> SVSFYEIANGNEVHTGSLNMTANPTSHELNVSAVLAAAKAKYAAHQLENGASNGASVAVTTDVKDLTDQLTKAGIKVDPLGNFQAQASFSFNLAAKSAQNAATATLPITVSVAN

S-layer proteins (SLPs) are self-assembling, crystalline proteins coating the cell surfaces of many prokaryotes. We determined the atomic resolution structures of all functional domains (I-III from N- to C-termini) present in the three S-layer proteins SlpA_ac, SlpX_ac, and SlpA_amy. The Lactobacillus S-layers are anchored to the cell wall through interaction with teichoic acids (TA), either lipoteichoic acid (LTA) or wall teichoic acid (WTA).

The arrangement and architecture of SlpA_ac and SlpA_amy are highly similar. The N-terminal part, exhibiting the first two domains (SlpA_I and SlpA_II), is known to be responsible for the self-assembly of the S-layer protein into a regular lattice. The crystal structures of SlpA from L. acidophilus and L. amylovorus and observed crystal contacts reveal the self-assembly formation. One basic tile is composed of the homodimer of the full-length SlpA, dimerized at the SlpA_II domain. The self-assembly region (SA) is formed by domains SlpA_I and SlpA_II, building a 2D crystalline network that forms the exposed surface of the SlpA layer.>[5x]MYSTAVLLNKISPTRDGQTMTLADLQYLSFSELRKIFDDQLSWGEARHLYHETIEQKKNNRLLEARIFTRANPQLSGAIRLGIERDSVSRSYDEMFGARSSSFVKPGSVASMFSPAGYLTELYREAKDLHFSSSAYHLDNRRPDLADLTLSQSNMDTEISTLTLSNELLLEHITRKTGGDSDALMESLSTYRQAIDTPYHQPYETIRQVIMTHDSTLSALSRNPEVMGQAEGASLLAILANISPELYNILTEEITEKNADALFAQNFSENITPENFASQSWIAKYYGLELSEVQKYLGMLQNGYSDSTSAYVDNISTGLVVNNESKLEAYKITRVKTDDYDKNINYFDLMYEGNNQFFIRANFKVSREFGATLRKNAGPSGIVGSLSGPLIANTNFKSNYLSNISDSEYKNGVKIYAYRYTSSTSATNQGGGIFTFESYPLTIFALKLNKAIRLCLTSGLSPNELQTIVRSDNAQGIINDSVLTKVFYTLFYSHRYALSFDDAQVLNGSVINQYADDDSVSHFNRLFNTPPLKGKIFEADGNTVSIDPDEEQSTFARSALMRGLGVNSGELYQLGKLAGVLDAQNTITLSVFVISSLYRLTLLARVHQLTVNELCMLYGLSPFNGKTTASLSSGELPRLVIWLYQVTQWLTEAEITTEAIWLLCTPEFSGNISPEISNLLNNLRPSISEDMAQSHNRELQAEILAPFIAATLHLASPDMARYILLWTDNLRPGGLDIAGFMTLVLKESLNANETTQLVQFCHVMAQLSLSVQTLRLSEAELSVLVISGFAVLGAKNQPAGQHNIDTLFSLYRFHQWINGLGNPGSDTLDMLRQQTLTADRLASVMGLDISMVTQAMVSAGVNQLQCWQDI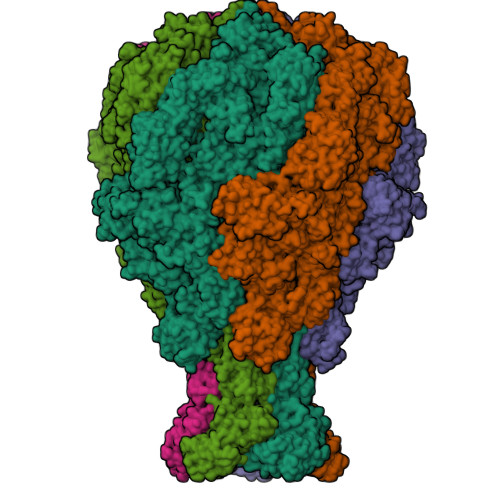NTVLQWIDVASALHTMPSVIRTLVNIRYVTALNKAESNLPSWDEWQTLAENMEAGLSTQQAQTLADYTAERLSSVLCNWFLANIQPEGVSLHSRDDLYSYFLIDNQVSSAIKTTRLAEAIAGIQLYINRALNRIEPNARADVSTRQFFTDWTVNNRYSTWGGVSRLVYYPENYIDPTQRIGQTRMMDELLENISQSKLSRDTVEDAFKTYLTRFETVADLKVVSAYHDNVNSNTGLTWFVGQTRENLPEYYWRNVDISRMQAGELAANAWKEWTKIDTAVNPYKDAIRPVIFRERLHLIWVEKEEVAKNGTDPVETYDRFTLKLAFLRHDGSWSAPWSYDITTQVEAVTDKKPDTERLALAASGFQGEDTLLVFVYKTGKSYSDFGGSNKNVAGMTIYGDGSFKKMENTALSRYSQLKNTFDIIHTQGNDLVRKASYRFAQDFEVPASLNMGSAIGDDSLTVMENGNIPQITSKYSSDNLAITLHNAAFTVRYDGSGNVIRNKQISAMKLTGVDGKSQYGNAFIIANTVKHYGGYSDLGGPITVYNKTKNYIASVQGHLMNADYTRRLILTPVENNYYARLFEFPFSPNTILNTVFTVGSNKTSDFKKCSYAVDGNNSQGFQIFSSYQSSGWLDIDTGINNTDIKITVMAGSKTHTFTASDHIASLPANSFDAMPYTFKPLEIDASSLAFTNNIAPLDIVFETKAKDGRVLGKIKQTLSVKRVNYNPEDILFLRETHSGAQYMQLGVYRIRLNTLLASQLVSRANTGIDTILTMETQRLPEPPLGEGFYATFVIPPYNLSTHGDERWFKLYIKHVVDNNSHIIYSGQLTDTNINITLFIPLDDVPLNQDYHAKVYMTFKKSPSDGTWWGPHFVRDDKGIVTINPKSILTHFESVNVLNNYSAPMDFNSASALYYWELFYYTPMMCFQRLLQEKQFDEATQWINYVYNPAGYIVNGEIAPWIWNCRPLEETTSWNANPLDAIDPDAVAQNDPMHYKIATFMRLLDQLILRGDMAYRELTRDALNEAKMWYVRTLELLGDEPEDYGSQQWAAPSLSGAASQTVQAAYQQDLTMLGRGGVSKNLRTANSLVGLFLPEYNPALTDYWQTLRLRLFNLRHNLSIDGQPLSLAIYAEPTDPKALLTSMVQASQGGSAVLPGTLSLYRFPVMLERTRNLVAQLTQFGTSLLSMAEHDDADELTTLLLQQGMELATQSIRIQQRTVDEVDADIAVLAESRRSAQNRLEKYQQLYDEDINHGEQRAMSLLDAAAGQSLAGQVLSIAEGVADLVPNVFGLACGGSRWGAALRASASVMSLSATASQYSADKISRSEAYRRRRQEWEIQRDNADGEVKQMDAQLESLKIRREAAQMQVEYQETQQAHTQAQLELLQRKFTNKALYSWMRGKLSAIYYQFFDLTQSFCLMAQEALRRELTDNGVTFIRGGAWNGTTAGLMAGETLLLNLAEMEKVWLERDERALEVTRTVSLAQFYQALSSDNFNLTEKLTQFLREGKGNVGASGNELKLSNRQIEASVRLSDLKIFSDYPESLGNTRQLKQVSVTLPALVGPYEDIRAVLNYGGSIVMPRGCSAIALSHGVNDSGQFMLDFNDSRYLPFEGISVNDSGSLTLSFPDATDRQKALLESLSDIILHIRYTIRSENLYFQGDYKDDDDKLEHHHHHH>GSHMEEKRLSAKKGLPPGTLVYTGKYREDFEIEVMNYSIEEFREFKTTDVESVLPFRDSSTPTWINITGIHRTDVVQRVGEFFGIHPLVLEDILNVHQRPKVEFFENYVFIVLKMFTYDKNLHELESEQVSLILTKNCVLMFQEKIGDVFDPVRERIRYNRGIIRKKRADYLLYSLIDALVDDYFVLLEKIDDEIDVLEEEVLERPEKETVQRTHQLKRNLVELRKTIWPLREVLSSLYRDVPPLIEKETVPYFRDVYDHTIQIADTVETFRDIV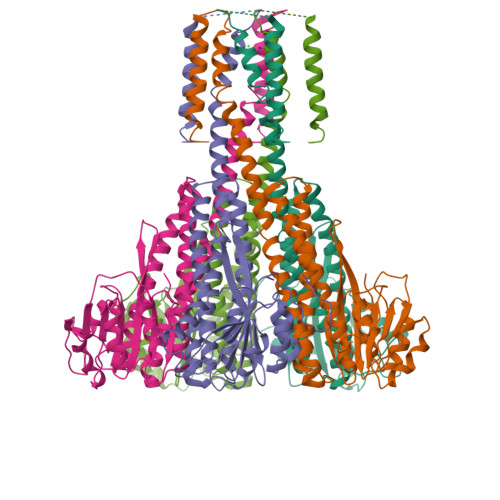SGLLDVYLSSVSNKTNEVMKVLTIIATIFMPLTFIAGIYGMNFEYMPELRWKWGYPVVLAVMGVIAVIMVVYFKKKKWL[5x]>MWSHPQFEKGSGGSGMSAVSGFTPSGQKRSLAELLDGRVKRLDRKSNNSVLQEAALYLLSCNQDVSQFLSEVEAPPYKKTCNPENPVSIKSRMPSAAFVGSTLKDQASCLKISPGILTAKAAVANIQQICQACGDSSAVLNPEQREKLCSLLKTLKILLAENCFCRSLFCKEIWIHRPPLVFEAVWHLHNEGIVCLDEILESCKDTISAVDWLFSEMCSLCLYIDNSSLAGDLAEKMISDFQALLVENSFRRSSATERILEQHKTEEICLSILDKLLSWLLDAVSVEKSDKSSAEQHWLSAFEVHRYRARVVPESIEQFFIHTLTQVLTFKPKLKVSDAIQCQANWSFVKTSTLLTDLYRKLFVALSAEKLIAHIQLVLDTQEVNWHHVLTCVSCLVICLPEAQQLIKDLLCRLLTHAFESYELEGMITAFLIVRQAALEGPAAFVSYTEWFKCTFGAANSYHGNSKKSLVFLLKFLSDIVPFEAPQYLKVHVLHPPFVPTKYRPLLMEYISLAKTRLTDMKVSIEDMGLYEDLSARSNKVQPESQAHQDVEKALNIFENTGKIPASVMEASIFRRPYFTSRFLPALLTPRVLPAAPDALMLLIDSMKRADKIPTNMFNAYIEACEQEKLRKQKGRQQMDQSLPDEPLGILQSALSDLRPLVTDANKYEDVSAQVAVISEKLIAVMGEQKVDDDQVAAKFLKLEDGAQLDIQEQTVADLLLTCFCQCLIAASGTNPPDRQGQWPTLYVKMLCGHQWAFAAVLRRMLQLLRFQAPFLKDSHIVGLAAFSIHLHECQPSLQFLITGVQNLEHYWENLLNLLCSDSVGVCLKLCTAAISYAFCRFSELHQDIFSGCVPPLFLRKLQYLVPRLIWETRGEVIRDDEEADSPLNWNLYALAGWKEAALSLWNQNRLQGLLREKSFQVTFMDWLLWEMTLKSNNDVLCDTDRQEYQRWAVNHYLSESSVVGGCNGDLERGCITIAEAVLQFSNRHIQHSEWESRNISMLKSHTGLGDILCRLQELICDIVTSHHQKGRRHFFFAIFYQRLELHKGKKELSNHLSKQGVLEMCCRILLGLPPLFLINTPSEKGIRTLGSEDFWQFVNKELKNLGPRGYALPYNITAHFFRGVISASVQCKDSSEAVNSILSATYSTCPALLISAAVGWPQLDPVLRSQWCSLFGVDLPKELRTLREQQASVDSCLSQGEKLSLSCTPWLSAAFLYSTVQRKKLPCSRMLEILDGLSSNFSMVLISLLFFSVMDIIYMFLKDGRKHKDLLENCVHIIHCLEQKGETWVWLFQMTDERKPELGLHLHRAASDVFLNLMPFAFFWLVPSLQLEQVVQQQDFLVIALDMYHKFLQLFVDGSPLSSLSAKSHHLDSHDVFTCGRQFLLCCVPKCQKPNSAILKKMLESWEEHDPELAAVLTRSFKAPDDYDDLFFEPVF[2x]

The FA pathway is triggered by stalled DNA replication forks at ICLs, leading to the activation of the FA core ubiquitin ligase complex. However, the FANCA–FANCG–FAAP20 (AG20) subcomplex is essential for monoubiquitination of FANCD2 in vivo. FANCA and FANCG are critical for the localization of the FANC core complex. To understand the basis of the FA-associated FANCA mutations, we determined the cryo-electron microscopy (EM) structures of Xenopus laevis FANCA alone at 3.35 Å and 3.46 Å resolution and two distinct FANCA–FANCG complexes at 4.59 and 4.84 Å resolution, respectively.

One of the major classes corresponds to the dimer of the CTD of FANCA. The two structures of FANCA alone show that the FANCA CTD folds into an arc-shaped solenoid structure, which forms a pseudo-symmetric dimer. The side chains of FANCA are well-defined in the 3.35 Å EM density map, and clusters of bulky hydrophobic side chains unambiguously guided the tracing of residues 631–1370 (helix H3A to helix H13B). The FANCA CTD structure consists of a chimera of 14 HEAT repeats and three helical motifs (HMs) with two to four helices. The convex surface forms a wide and shallow groove (44 Å width, 35 Å length, 6 Å depth), through which the extensive dimer interface (6238 Å2) is created. The two FANCA CTDs interact in a head-to-tail manner, in which the arcC subdomain of FANCA’ CTD (green) interacts with the arcN subdomain of FANCA CTD (orange). The dimeric interface between the two FANCA CTD molecules includes an extended network of interactions involving more than 40 H-bonds, 10 ion-pairs and extensive hydrophobic and van der Waals contacts. At the center of the dimer, two parallel H8B helices run along the 2-fold rotation axis. Two Cys pairs (C999-C999 and C1006-C1006) are in close proximity, consistent with the results of the intermolecular crosslinking analysis using hydrogen peroxide and bis-maleimidoethane. The FANCA CTD structure reveals a long path decorated with a cluster of positively charged residues, providing a rationale for how FANCA might interact with DNA.> MKHHHHHHMKQNSPLDEENLTQENQDRGTHVDRGLASANVDFAFSLYKQLVLKAPDKNVIFSPVSISTALAFLSLGAHNTTLTEILKGLKFNLTETSEAEIHQSFQHLLRTLNQSSDELQLSMGNAMFVKEQLSLLDRFTEDAKRLYGSEAFATDFQDSAAAKKLINDYVKNGTRGKITDLIKDLDSQTMMVLVNYIFFKAKFEMPFDPQDTHQSRFYLSKKKYVMVPMMSLHHLTIPYFRDEELSCTVVQLNYTGNASALFILPDQDKMEEVEAMLSQETLSRFFESLEFREIGELYLPKFSISRDYNLNDILLQLGIEEAFTSKADLSGITGARNLAVSQVVHKAVLDVFEEGTERSAATALEVLFQ;> GPLVETRTIVRFNRPFLM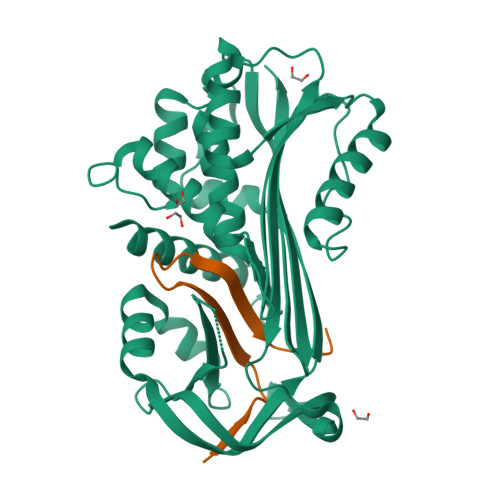IIVDNFTWSIFFMSKVTNPKQA> SSNDNIELVDFQNIMFYGDAEVGDNQQPFTFILDTGSANLWVPSVKCTTAGCLTKHLYDSSKSRTYEKDGTKVEMNYVSGTVSGFFSKDLVTVGNLSLPYKFIEVIDTNGFEPTYTASTFDGILGLGWKDLSIGSVDPIVVELKNQNKIENALFTFYLPVHDKHTGFLTIGGIEERFYEGPLTYEKLNHDLYWQITLD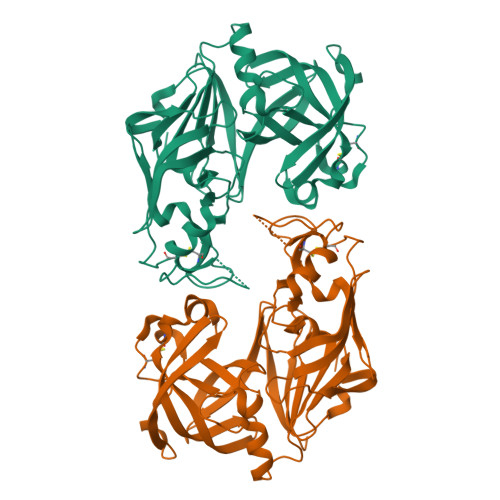AHVGNISLEKANCIVDSGTSAITVPTDFLNKMLQNLDVIKVPFLPFYVTLCNNSKLPTFEFTSENGKYTLEPEYYLQHIEDVGPGLCMLNIIGLDFPVPTFILGDPFMRKYFTVFDYDNHSVGIALAKKNL KCa2.1, KCa2.2, KCa2.3, and KCa3.1, also known as SK1–4 (or SK1–3 and IK1), are small- (KCa2.1–2.3) or intermediate-conductance (KCa3.1) potassium channels encoded by the KCNN genes. These homotetrameric potassium channels constitutively bind the calcium-binding protein calmodulin (CaM) in their cytoplasmic regions, and calcium binding to channel-associated CaM is thought to induce a conformational change that leads to channel opening. By effluxing potassium ions, KCa3.1 maintains a negative membrane potential necessary for sustained calcium influx via calcium release-activated channels (CRACs) and for subsequent cytokine production. The cytoplasmic domain contains a CaM-binding region followed by a predicted coiled-coil region near the C-terminus, which is important for proper processing and trafficking of the channel.

To characterize structurally the C-terminal coiled-coil region in KCa3.1 (KCa3.1-CC), we determined its crystal structure at 1.75-Å resolution. The structure reveals a parallel four-helix bundle, consistent with the tetrameric nature of the channel. The space group of the tetragonal crystals is P4212, and the asymmetric unit comprises two KCa3.1-CC molecules. In the structure of copper-containing KCa3.1-CC, the crystallographic four-fold axis generates two parallel four-helix bundles comprising four (identical) copies of each of the two KCa3.1-CC protomers in the asymmetric unit. The packing within the crystal is diagrammed in S1 Fig. The root-mean-square deviation (rmsd) of Cα atoms (residues 378–411) for the two copies of KCa3.1-CC in the asymmetric unit is 0.49 Å. As expected, based on coiled-coil prediction software, His389 occupies an inward-facing ‘a’ position in the heptad repeat of the coiled-coil/four-helix bundle. In the copper-containing structure, a copper ion is positioned on the four-fold axis, ligated by the NE2 nitrogen atom (also known as N3) of the imidazole ring from each of the four copies of His389, with an N3-Cu distance of 2.1 Å. An axial water molecule, at 2.5 Å on the N-terminal side, completes the square-pyramidal coordination. Based on the coordination geometry, the copper ion is Cu(II). In the partially refined apo structure, the side chain of His389 points away from the center of the four-helix bundle (data not shown).

>[2x]GSMILYDLQQNLSSSHRALEKQIDTLAGKLDALTELLSTALG{(3R,4S)-1-[(4-amino-5H-pyrrolo[3,2-d]pyrimidin-7-yl)methyl]-4-hydroxypyrrolidin-3-yl}-L-methionine | C16 H24 N6 O3 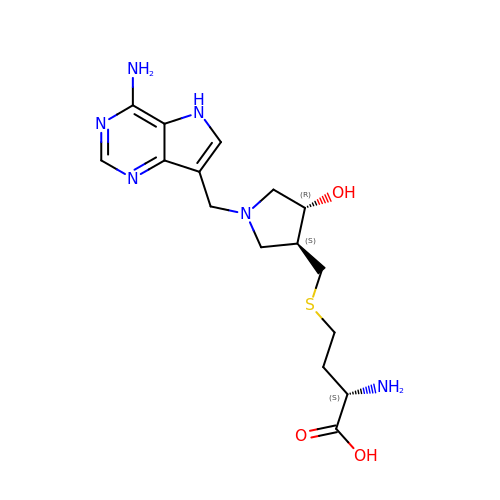S | DQWJHDQQDUJDLQ-WOPDTQHZSA-N> MNENI;> MAIYADNSYSIGNTPLVRLKHFGHNGNVVVKIEGRNPSYSVKCRIGANMVWQAEKDGTLTKGKEIVDATSGNTGIALAYVAAARGYKITLTMPETMSLERKRLLCGLGVNLVLTEGAKGMKGAIAKAEEIVASDPSRYVMLKQFENPANPQIHRETTGPEIWKDTDGKVDVVVAGVGTGGSITGISRAIKLDFGKQITSVAVEPVESPVISQTLAGEEVK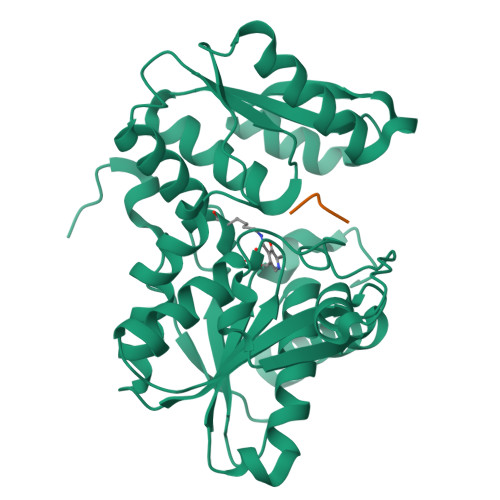PGPHKIQGIGAGFIPKNLDLSIIDRVETVDSDTALATARRLMAEEGILAGISSGAAVAAADRLAKLPEFADKLIVVILPSASERYLSTALFEGIEG> PEPWFFKNLSRKDAERQLLAPGNTHGSFLIRESESTAGSFSLSVRDFDQNQGEVVKHYKIRNLDNGGFYISPRITFPGLHELVRHY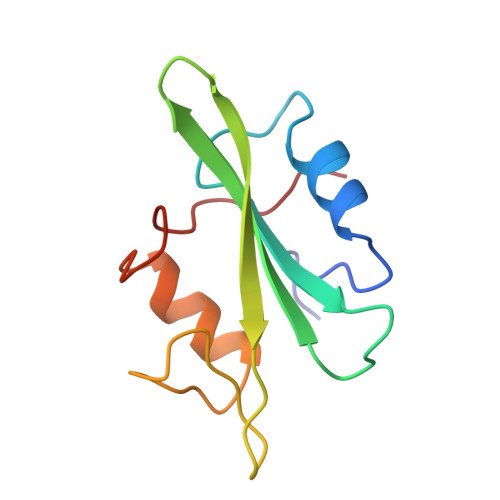TNASDGLCTRLSRPCQT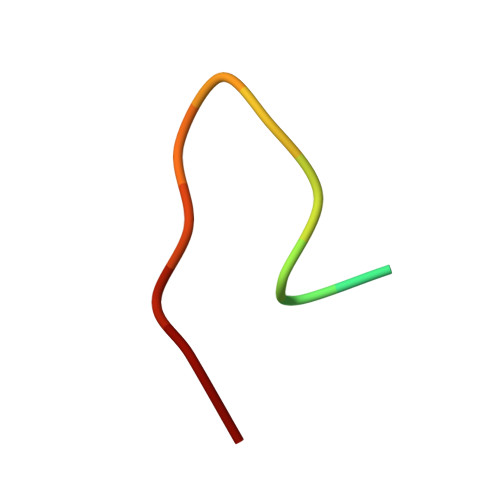> TRYWNAKMLPFAFGA>MAIT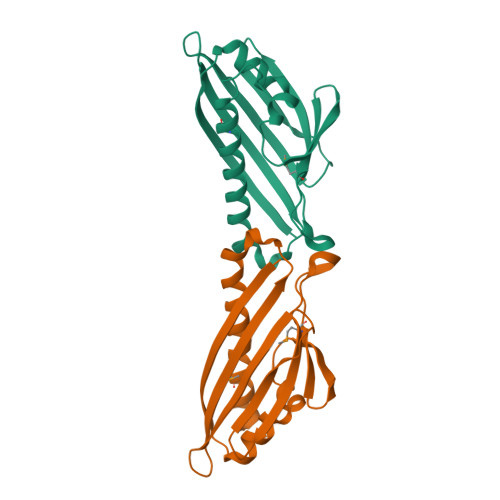VSIELNRDLEIPASYDEVFDLLADVPKSASHFPKVDKLVDLGNNAYRWEMEKVGVDKHAIQSVYACTYHADKEAGKITWSPIKGEGNGVVSGSWTLSAKGDNATAVKFQTSAELTVPLPSLLKLAISPVIKHEFNSLVDTYMANLKKAFLEHHHHHH[2x]2'-deoxy-2'-triaza-1,2-dien-2-ium-1-yl-uridine-5'-monophosphate | C9 H13 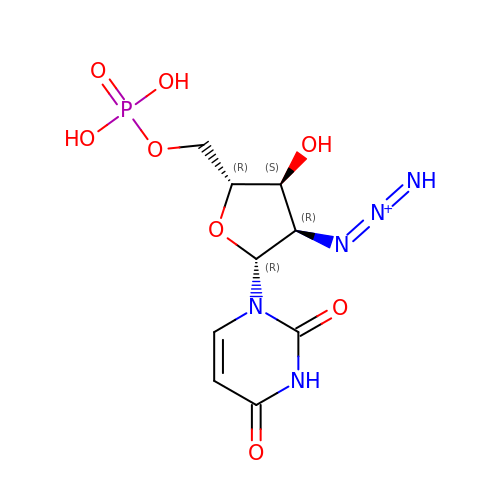N5 O8 P | FKBDCNLBVFTTRL-XVFCMESISA-O> NEQSGKSQTVIV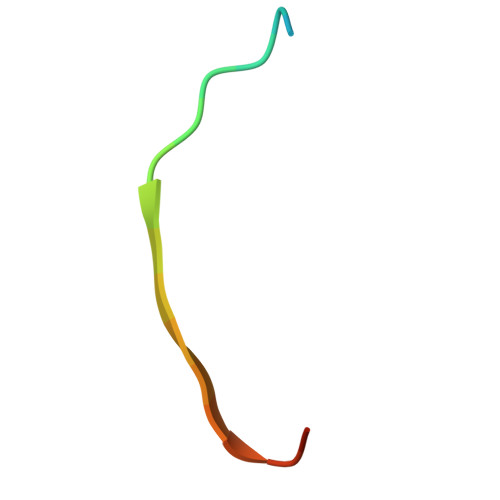GSWGAKVS Resistance nodulation and cell division (RND) efflux pumps are secondary active antiporters that are ubiquitous across all domains of life. As part of tripartite multidrug efflux systems in Gram-negative bacteria, they span the entire cell envelope and export a broad variety of structurally and chemically unrelated toxic substrates. During drug efflux, AcrB undergoes a functional rotation where each of the three protomers sequentially cycles through the conformational states loose (L), tight (T) and open (O). Substrates can enter the PD through several channels and bind to the access pocket (AP) in the L state and the deep binding pocket (DBP) in the T state.

Further, we reconstituted OqxB in SP-ND to assess its distribution of conformational states in a detergent free environment with cryo-EM. In contrast to all AcrB samples, that contained a mixture of several trimeric states, OqxB showed a homogeneous structure with all particle classes representing the same state. Based on the electron density map of the OqxB trimer, a structural model was built with 2.8 Å global resolution. The three individual protomers in the OqxB trimer adopt a highly similar conformation with an all-atom RMSD between the individual chains of ≤ 0.8. However, in all three monomers of OqxB all channels leading to the PD, including the exit tunnel, are very narrow throughout their entire length with a bottleneck radius between 1.1 Å and 1.5 Å. These channels are too narrow to fit any known OqxB substrate. Thus, the cryo-EM structure of OqxB has the typical architecture of the O state, but with a closed exit tunnel and will hereafter be referred to as O*O*O* state. In contrast to the O state observed in the crystallographic TTO structure, the O* state of OqxB has a pronounced shift in the PN1 subdomain, which is likely the reason for the closed configuration of the exit channel. The O* state might represent a local energy minimum in the OqxB structure which leads to the formation of O*O*O* in the absence of a substrate. On the other side of the spectrum, OqxB adopts a single trimer conformation, the O*O*O* state, in which all binding pockets and entrance channels are closed.

>[3x]MDFSRFFIDRPIFAAVLSILIFITGLIAIPLLPVSEYPDVVPPSVQVRAEYPGANPKVIAETVATPLEEAINGVENMMYMKSVAGSDGVLVTTVTFRPGTDPDQAQVQVQNRVAQAEARLPEDVRRLGITTQKQSPTLTLVVHLFSPNGKYDSLYMRNYATLKVKDELARLPGVGQIQIFGSGEYAMRVWLDPNKVAARGLTASDVVTAMQEQNVQVSAGQLGAEPLPQESDFLISINAQGRLHTEEEFGNIILKTAQDGSLVRLRDVARIEMGSGSYALRSQLNNKDAVGIGIFQSPGANAIDLSNAVRAKMAELATRFPEDMQWAAPYDPTVFVRDSIRAVVQTLLEAVVLVVLVVILFLQTWRASIIPLIAVPVSVVGTFSILYLLGFSLNTLSLFGLVLAIGIVVDDAIVVVENVERNIEEGLAPLAAAHQAMREVSGPIIAIALVLCAVFVPMAFLSGVTGQFYKQFAVTIAISTVISAINSLTLSPALAALLLKPHGAKKDLPTRLIDRLFGWIFRPFNRFFLRSSNGYQGLVSKTLGRRGAVFAVYLLLLCAAGVMFKVVPGGFIPTQDKLYLIGGVKMPEGSSLARTDAVIRKMSEIGMNTEGVDYAVAFPGLNALQFTNTPNTGTVFFGLKPFDQRKHTAAEINAEINAKIAQIQQGFGFSILPPPILGLGQGSGYSLYIQDRGGLGYGALQSAVNAMSGAIMQTPGMHFPISTYQANVPQLDVQVDRDKAKAQGVSLTELFGTLQTYLGSSYVNDFNQFGRTWRVMAQADGPYRESVEDIANLRTRNNQGEMVPIGSMVNISTTYGPDPVIRYNGYPAADLIGDADPRVLSSSQAMTHLEELSKQILPNGMNIEWTDLSFQQATQGNTALIVFPVAVLLAFLVLAALYESWTLPLAVILIVPMTMLSALFGVWLTGGDNNVFVQVGLVVLMGLACKNAILIVEFARELEIQGKGIMEAALEACRLRLRPIVMTSIAFIAGTIPLILGHGAGAEVRGVTGITVFSGMLGVTLFGLFLTPVFYVTLRKLVTRRKPVQEDLPAHHHHHH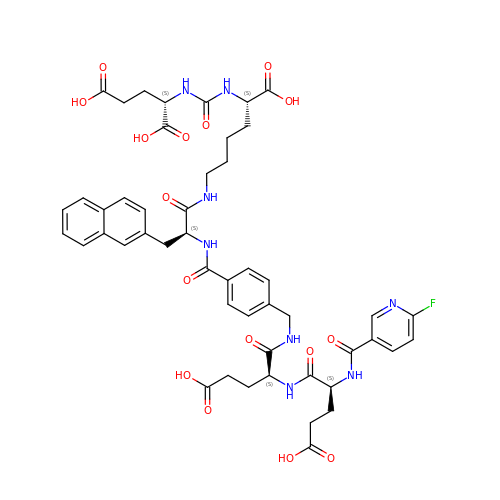(2~{S})-2-[[(2~{S})-6-[[(2~{S})-2-[[4-[[[(2~{S})-2-[[(2~{S})-2-[(6-fluoranylpyridin-3-yl)carbonylamino]-5-oxidanyl-5-oxidanylidene-pentanoyl]amino]-5-oxidanyl-5-oxidanylidene-pentanoyl]amino]methyl]phenyl]carbonylamino]-3-naphthalen-2-yl-propanoyl]amino]-1-oxidanyl-1-oxidanylidene-hexan-2-yl]carbamoylamino]pentanedioic acid | C49 H55 F N8 O16 | RFFFFGRYVZESLB-LTLCPEALSA-N> MSEAEARPTNFIRQIIDEDLASGKHTTVHTRFPPEPNGYLHIGHAKSICLNFGIAQDYKGQCNLRFDDTNPVKEDIEYVESIKNDVEWLGFHWSGNVRYSSDYFDQLHAYAIELINKGLAYVDELTPEQIREYRGTLTQPGKNSPYRDRSVEENLALFEKMRAGGFEEGKACLRAKIDMASPFIVMRDPVLYRIKFAEHHQTGNKWCIYPMYDFTHCISDALEGITHSLRTLEFQDNRRLYDWVLDNITIPVHPRQ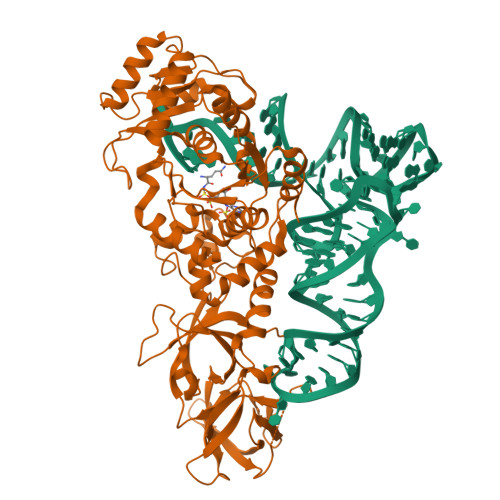YEFSRLNLEYTVMSKRKLNLLVTDKHVEGWDDPRMPTISGLRRRGYTAASIREFCKRIGVTKQDNTIEMASLESCIREDLNENAPRAMAVIDPVKLVIENYQGEGEMVTMPNHPNKPEMGSRQVPFSGEIWIDRADFREEANKQYKRLVLGKEVRLRNAYVIKAERVEKDAEGNITTIFCTYDADTLSKDPADGRKVKGVIHWVSAAHALPVEIRLYDRLFSVPNPGAADDFLSVINPESLVIKQGFAEPSLKDAVAGKAFQFEREGYFCLDSRHSTAEKPVFNRTVGLRDTLEHHHHHH> MDYMNL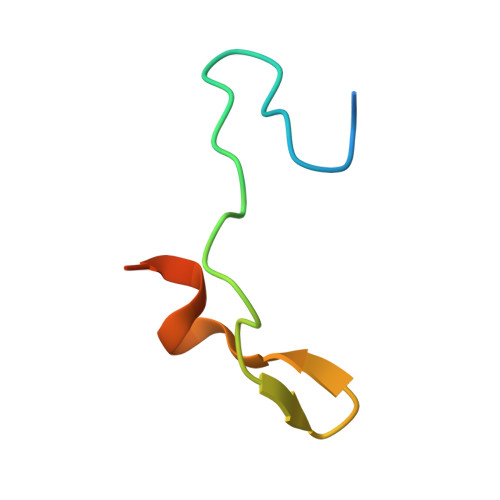GVKSRKTGLTVNKTVQKDEYSMENLNDFFKDEQDS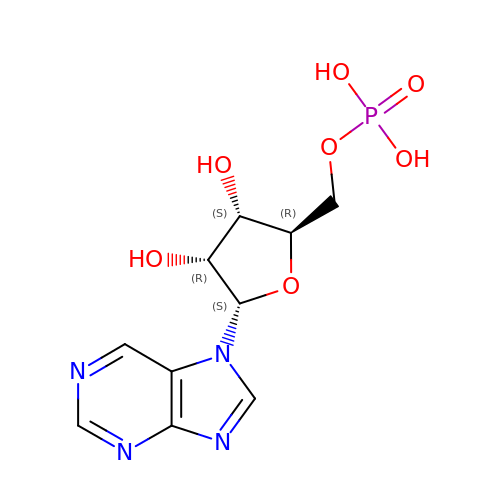7-ALPHA-D-RIBOFURANOSYL-PURINE-5'-PHOSPHATE | C10 H13 N4 O7 P | NICKPTPNIMHUHB-DQUBFYRCSA-N>[2x]GMQENTRLRIAIQKSGRLSKESIELLSECGVKMHIHEQSLIAFSTNLPIDILRVRDDDIPGLIFDGVVDLGIIGENVLEENELERQSLG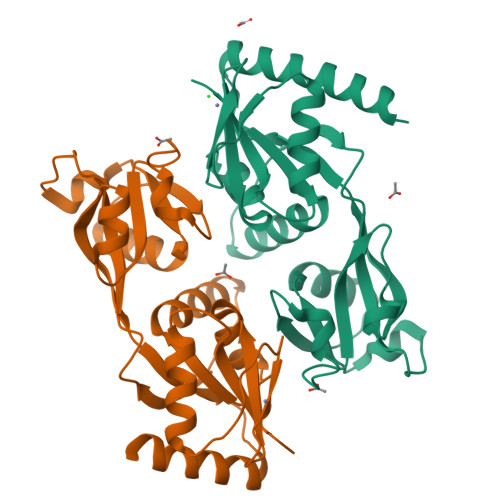ENPSYKLLKKLDFGYCRLSLALPQENKFQNLKDFEGLRIATSYPQLLKRFMKENGINYKNCTLTGSVEVAPRANLADAICDLVSSGATLQANNLKEVKVIYESRACLIQKENALSKEKQALVDKIMLRVAGVMQARE> MDDISPSELKTILHSKRANLYYLQHCRVLVNGGRVEYVTDEGRHSHYWNIPIANTTSLLLGTGTSITQAAMRELARAGVLVGFCGGGGTPLFSANEVDVEVSWLTPQSEYRPTEYLQRWVGFWFDEEKRLVAARHF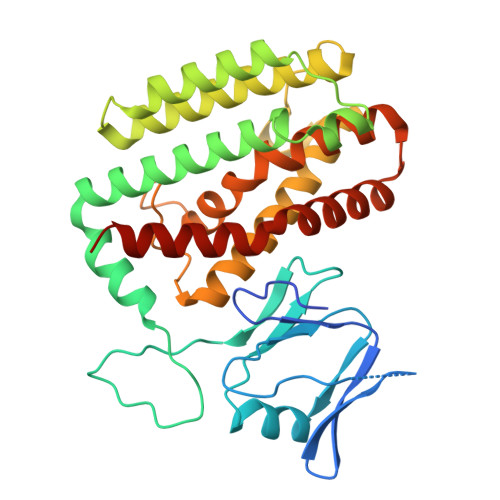QRARLERIRHSWLEDRVLRDAGFAVDATALAVAVEDSARALEQAPNHEHLLTEEARLSKRLFKLAAQATRYGEFVRAKRGSGGDPANRFLDHGNYLAYGLAATATWVLGIPHGLAVLHGKTRRGGLVFDVADLIKDSLILPQAFLSAMRGDEEQDFRQACLDNLSRAQALDFMIDTLKDVAQRSTVSA>[2x]ARLGARPCGLRE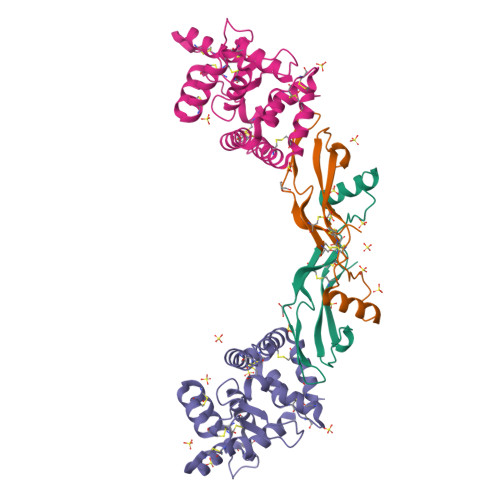LEVRVSELGLGYASDETVLFRYCAGACEAAARVYDLGLRRLRQRRRLRRERVRAQPCCRPTAYEDEVSFLDAHSRYHTVHELSARECACV;>GTGADPVVSAKSNHCLDAAKACNLNDNCKKLRSSYISICNREISPTERCNRRKCHKALRQFFDRVPSEYTYRMLFCSCQDQACAERRRQTILPSCSYEDKEKPNCLDLRGVCRTDHLCRSRLADFHANCRASYQTVTSCPADNYQACLGSYAGMIGFDMTPNYVDSSPTGIVVSPWCSCRGSGNMEEECEKFLRDFTENPCLRNAIQAFGNGTDVN[2x]>DIPIGQKMTGKMTYYTDKGYGACGTPIDASSQDLVAIPAAWWTTPNPNNDPLCRGVSVEVSYNGRTIRVPVRDKCPSCDRTHIDLSQAAFAKLAPLDRGVVNGITWK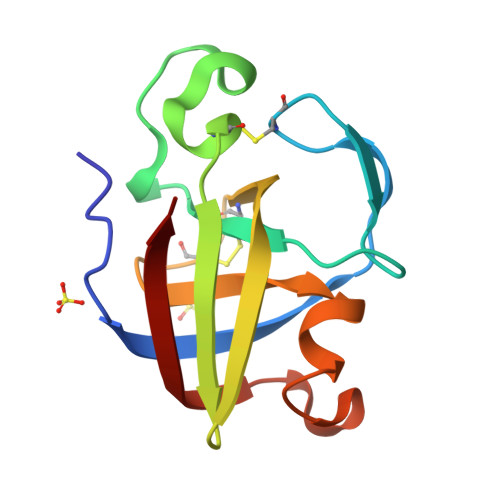FVR[2x]> AKPCTVSTTNATVDLGDLYSFSLMSAGAASAWHDVALELTNCPVGTSRVTASFSGAADSTGYYKNQGTAQNIQLELQDDSGNTLNTGATKTVQVDDSSQSAHFPLQVRAL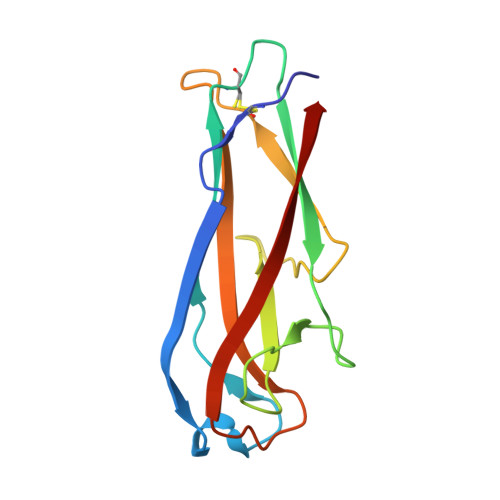TVNGGATQGTIEAVIEITYTYS[(2S,3R,4R,5R)-5-(6-aminopurin-9-yl)-3,4-bis(oxidanyl)oxolan-2-yl] 2-(1H-indol-3-yl)ethyl hydrogen phosphate | C19 H21 N6 O7 P | 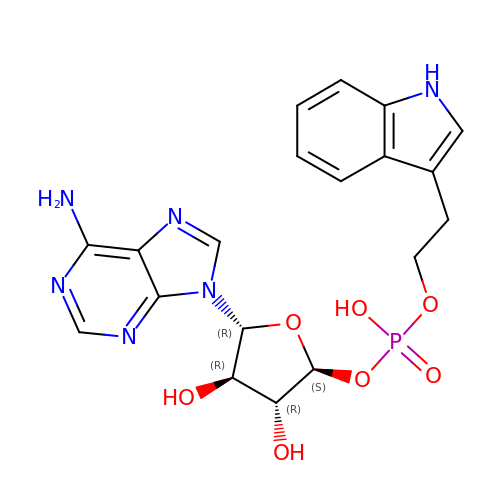OLRAQXYDQRFQTA-RGCFKVTRSA-N> CVTQLLKDTCFEGGDITTVFTPSAKYCQVVCTYHPRCLLFTFTAESPSEDPTRWFTCVLKDSVTETLPRVNRTAAISGYSFKQCSHQISACNKDIYVDLDMKGINYNSSVAKSAQECQERCTDDVHCHFFTYATRQFPSLEHRNICLLKHTQTGTPTRITKLDKVVSGFSLKSCALSNLACIRDIFPNTVFADSNIDSVMAPDAFVCGRICTHHPGC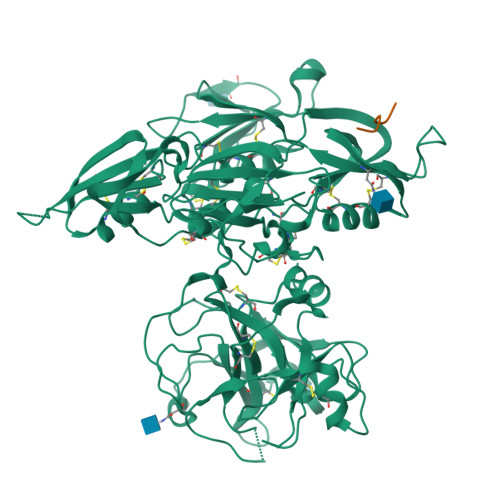LFFTFFSQEWPKESQRNLCLLKTSESGLPSTRIKKSKALSGFSLQSCRHSIPVFCHSSFYHDTDFLGEELDIVAAKSHEACQKLCTNAVRCQFFTYTPAQASCNEGKGKCYLKLSSNGSPTKILHGRGGISGYTLRLCKMDNECTTKIKPRIVGGTASVRGEWPWQVTLHTTSPTQRHLCGGSIIGNQWILTAAHCFYGVESPKILRVYSGILNQSEIKEDTSFFGVQEIIIHDQYKMAESGYDIALLKLETTVNYTDSQRPICLPSKGDRNVIYTDCWVTGWGYRKLRDKIQNTLQKAKIPLVTNEECQKRYRGHKITHKMICAGYREGGKDACKGDSGGPLSCKHNEVWHLVGITSWGEGCAQRERPGVYTNVVEYVDWILEKTQAV;> EFPDFP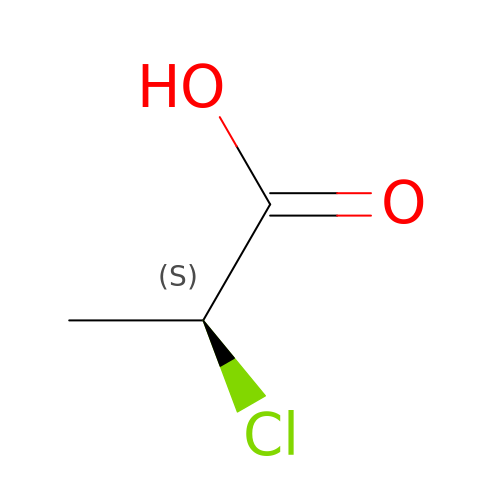(2S)-2-CHLOROPROPANOIC ACID | C3 H5 Cl O2 | GAWAYYRQGQZKCR-REOHCLBHSA-N> HHHHHHGSGTNVNDKVTASNFKLEKTTFDPNQSGNTFMAANFTVTDKVKSGDYFTAKLPDSLTGNGDVDYSNSNNTMPIADIKSTNGDVVAKATYDILTKTYTFVFTDYVNNKENINGQFSLPLFTDRAKAPKSGTYDANINIADEMFNNKITYN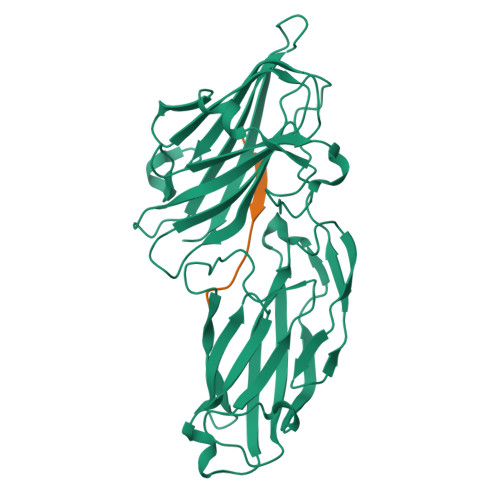YSSPIAGIDKPNGANISSQIIGVDTASGQNTYKQTVFVNPKQRVLGNTWVYIKGYQDKIEESSGKVSATDTKLRIFEVNDTSKLSESYYADPNDSNLKEVTDQFKNRIYYEHPNVASIKFGDITKTYVVLVEGHYDNTGKNLKTQVIQENVDPVTNRDYSIFGWNNENVVRYGGGSADGDSAV;> GSWNSGSSGTGSTGNQ(4R,7S)-7-hydroxy-1-(4-methoxybenzyl)-7-methyl-4,5,6,7-tetrahydro-1H-benzotriazol-4-yl propan-2-ylcarbamate | C19 H26 N4 O4 | 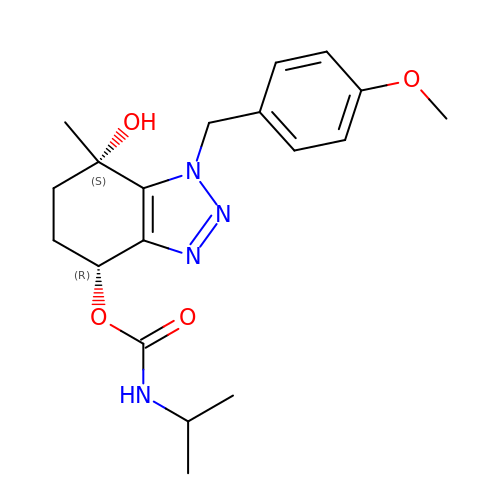CDAJJINZTVFCPA-BEFAXECRSA-N>LDVYVNFPADGHVREIAKTVLDGFDLHWYPDYYDAEAQVIKDRYVLGKRTKMIQAISAGVDHIDVNGIPENVVLCSNAGAYSISVAEHAFALLLAHAKNILENNELMKAGIFRQSPTTLLYGKALGILGYGGIGRRVAHLAKAFGMRVIAYTRSSVDQNVDVISESPADLFRQSDFVLIAIPLTDKTRGMVNSRLLANARKNLTIVNVARADVVSKPDMIGFLKERSDVWYLSDVWWNEPEITETNLRNAILSP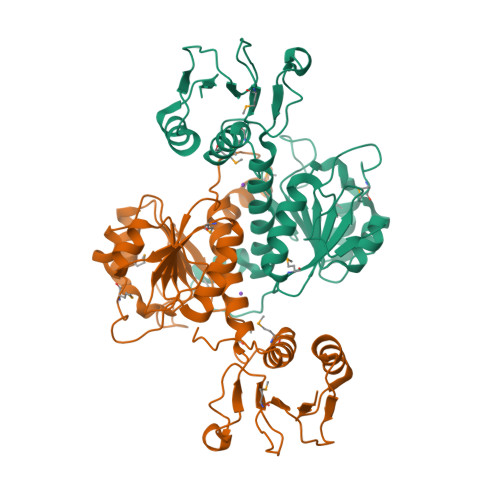HVAGGMSGEIMDIAIQLAFENVRNFFEGEGHHHHHH[2x]> MTEKEKMLAEKWYDANFDQYLINERARAKDICFELNHTRPSATNKRKELIDQLFQTTTDNVSISIPFDTDYGWNVKLGKNVYVNTNCYFMDGGQITIGDNVFIGPNCGFYTATHPLNFHHRNEGFEKAGPIHIGSNTWFGGHVAVLPGVTIGEGSVIGAGSVVTKDIPPHSLAVGNPCKVVRKI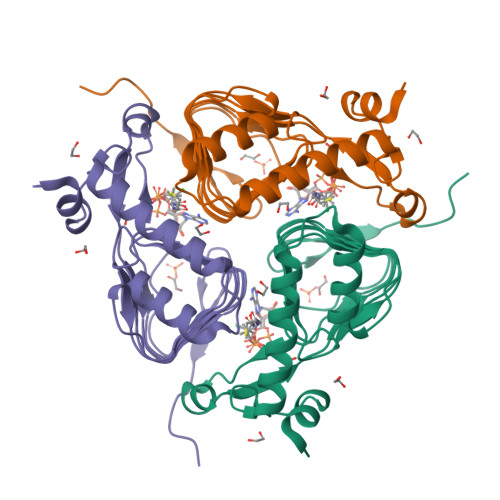DNDLPSETLNDETIK Though anhydrobiotic tardigrades (micro‐animals also known as water bears) possess many genes of secretory abundant heat soluble (SAHS) proteins unique to Tardigrada, their functions are unknown. Secretory abundant heat soluble (SAHS) protein is one of them and is constantly expressed at high levels in Ramazzottius varieornatus. A previous crystallographic study revealed that a SAHS protein (RvSAHS1) from one of the toughest tardigrades, Ramazzottius varieornatus, has a β‐barrel architecture similar to fatty acid binding proteins (FABPs) and two putative ligand binding sites (LBS1 and LBS2) where fatty acids can bind. However, some SAHS proteins such as RvSAHS4 have different sets of amino acid residues at LBS1 and LBS2, implying that they prefer other ligands and have different functions.

The RvSAHS4 structure was refined at 1.5 Å resolution. The overall structure of RvSAHS4 shared a typical FABP fold having an antiparallel β‐barrel composed of 10 β‐strands, and a helix‐turn‐helix lid between βA and βB. Helix αII in the RvSAHS4 structure had only a single turn and shorter than those in FABPs as is observed in RvSAHS1 structures. However, MolB in the RvSAHS4 structure had a 310 helix (η1) following αII and MolA also had a helix‐like structure in the same region [Fig. 1(C)]. While LBS1 in RvSAHS1 possesses an endogenous FA molecule originating from Escherichia coli in the crystal structure, no electron density corresponding to an FA molecule was observed around LBS1 in RvSAHS4. Residues located at LBS2 in RvSAHS4 were also distinct from those in RvSAHS1. LBS2 in RvSAHS4 was constituted by Cys120, Val142, Tyr144, and Gln153, which respectively correspond to Tyr117, Asp139, Tyr141, and Lys150 in RvSAHS1 [Fig. 2(B)]. Hydrophobic compounds such as FAs, bile acids, and retinoid, which are ligands for FABP family proteins, could not fit well into the electron density. Therefore, we modeled short PEG molecules contained in the crystallization solution (triethylene glycol in MolA and tetraethylene glycol in MolB) [Fig. 2(C), S2, Supporting Information]. The terminal oxygen atom of the PEG molecules could form hydrogen bonds with Thr129, Tyr75, and a nearby water molecule. Our observation that LBS1 in RvSAHS4 is blocked by Tyr65 and that PEG molecules were found at LBS2 suggests that RvSAHS4 mainly uses LBS2 to capture ligands.

>MGSSHHHHHHENLYFQSQWTGKPWLGKWESIDGTPENWEAFVKAANIPPKDQALYNGKQKTLLKYWKEAGEDHYHVQTSFPGTEHKMETSFKMGQEGTLSHDGVDLKYVCTEDGEQLITKINIPSKNQETIVTYTATGDDLEQTFTSNGVTGKRWYKKIHA[2x]>[4x]MEEAPLFPGESIKAIVKDVMYICPFMGAVSGTLTVTDFKLYFKNVERDPHFILDVPLGVISRVEKIGAQSHGDNSCGIEIVCKDMRNLRLAYKQEEQSKLGIFENLNKHAFPLSNGQALFAFSYKEKFPINGWKVYDPVSEYKRQGLPNESWKISKINSNYEFCDTYPAIIVVPTSVKDDDLSKVAAFRAKGRVPVLSWIHPESQATITRCSQPLVGPNDKRCKEDEKYLQTIMDANAQSHKLIIFDARQNSVADTNKTKGGGYESESAYPNAELVFLEIHNIHVMRESLRKLKEIVYPSIDEARWLSNVDGTHWLEYIRMLLAGAVRIADKIESGKTSVVVHSSDGWDRTAQLTSLAMLMLDSYYRTIKGFETLVEKEWISFGHRFALRVGHGNDNHADADRSPIFLQFVDCVWQMTRQFPSAFEFNELFLITILDHLYSCLFGTFLCNCEQQRFKEDVYTKTISLWSYINSQLDEFSNPFFVNYENHVLYPVASLSHLELWV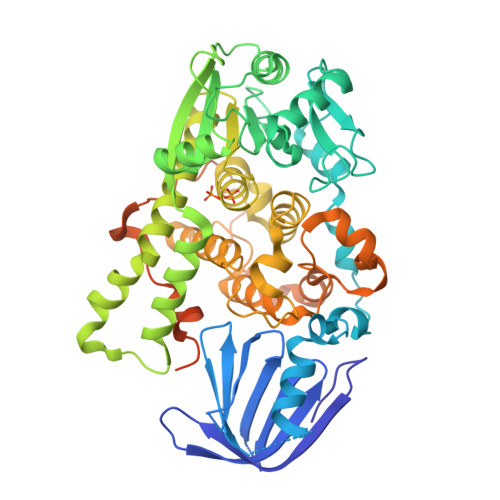NYYVRWNPRMRPQMPIHQNLKELLAVRAELQKRVEGLQREVATRAVSSSSERGSSPSHSATSVHTSV6-(3-METHYL-1,4-DIOXO-1,4-DIHYDRONAPHTHALEN-2-YL)HEXANOIC ACID | C17 H18 O4 | 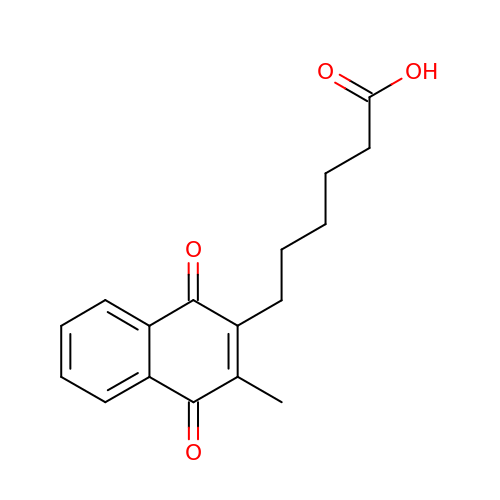ICGRXHWXPCXIKM-UHFFFAOYSA-N> MIFSVDKVRADFPVLSREVNGLPLAYLDSAASAQKPSQVIDAEAEFYR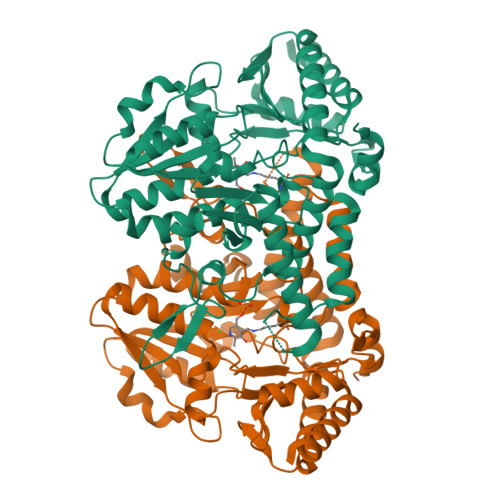HGYAAVHAGIHTLSAQATEKMENVRKRASLFINARSAEELVFVRGTTEGINLVANSWGNSNVRAGDNIIISQMEHHANIVPWQMLCARVGAELRVIPLNPDGTLQLETLPTLFDEKTRLLAITHVSNVLGTENPLAEMITLAHQHGAKVLVDGAQAVMHHPVDVQALDCDFYVFSGHKLYGPTGIGILYVKEALLQEMPPWEGGGSMIATVSLSEGTTWTKAPWRFEAGTPNTGGIIGLGAALEYVSALGLNNIAEYEQNLMHYALSQLESVPDLTLYGPQNRLGVIAFNLGKHHAYDVGSFLDNYGIAVRTGHHCAMPLMAYYNVPAMCRASLAMYNTHEEVDRLVTGLQRIHRLLG> SNAMDYQTIPSQGLSGEIC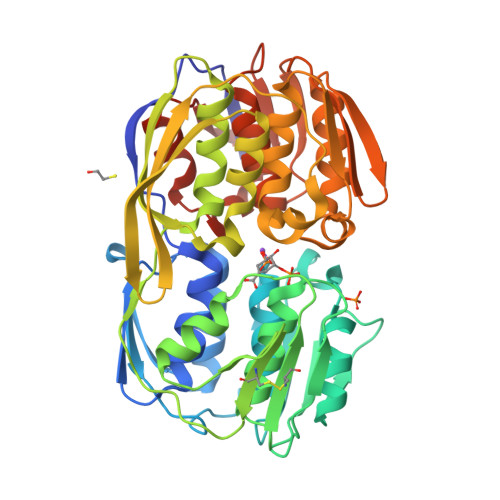VPGDKSISHRAVLLAAIAEGQTQVDGFLMGADNLAMVSALQQMGASIQVIEDENILVVEGVGMTGLQAPPEALDCGNSGTAIRLLSGLLAGQPFNTVLTGDSSLQRRPMKRIIDPLTLMGAKIDSTGNVPPLKIYGNPRLTGIHYQLPMASAQVKSCLLLAGLYARGKTCITEPAPSRDHTERLLKHFHYTLQKDKQSICVSGGGKLKANDISIPGDISSAAFFIVAATITPGSAIRLCRVGVNPTRLGVINLLKMMGADIEVTHYTEKNEEPTADITVRHARLKGIDIPPDQVPLTIDEFPVLLIAAAVAQGKTVLRDAAELRVKETDRIAAMVDGLQKLGIAAESLPDGVIIQGGTLEGGEVNSYDDHRIAMAFAVAGTLAKGPVRIRNCDNVKTSFPNFVELANEVGMNVKGVRGRGGF> APLNAARPAEERAALLAWVKERLHEEYGDQDPTPRRDPMHELISTILSQQTTHADEEAAYQELRTLGDWDAITLAPTDAVAH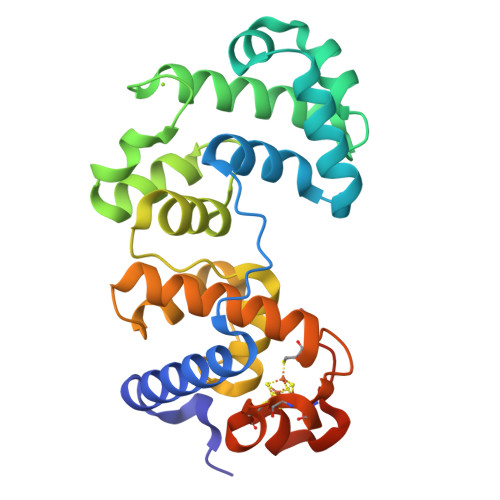AIRRSNYPESKAPRIQETLRRIKAAPGGYDLDFLRDLPVKDALKWLTDLPGVGVKTASLVLLFNYARPVFPVDTHVHRVSTRVGVIPRMGEQAAHRALLALLPPDPPYLYELHINFLSHGRQVCTWTRPKCGKCILRERCDAYALYGDKVPSFSEKPVKGEKPAKG>[2x]MAFCFGSFFSKYASSKSGSQARYRFLHSSAKIAAGATGALLLGGATVALCYFPSGRKVTEAPPFDVNSLRRDIEEILSEDMSKGPLFVRLAWHEAGSWDCRKKDGSPNSASMRFHPECSYAGNKGLDKGRNALESLKKKYPKISYADLWSFAAVVSIEAMGGPEIPWRWGRVDAKDGSVCGPDGRLPDASRMQDHVRDVFSRLGFNDEETVAL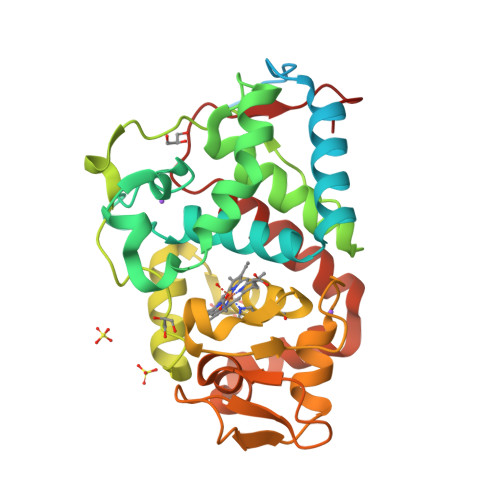IGAHTCGECHLENTGYVGPFTHDKYGFDNSFFTELFGNEWMLNPNVKKMQFMDKTTNRLMMLPADVSILLDDKYRSIAKKYADDNDYFCNAFSKAYQKLLEVGTTDLKSLPAESK> PSCVMDDFRDPQRWKECAKQGKMPCYFDLIEENVYLTERAKNKSHRDIKRMQCECTPLSKDERAQGEIACGEDCLNRLLMIECS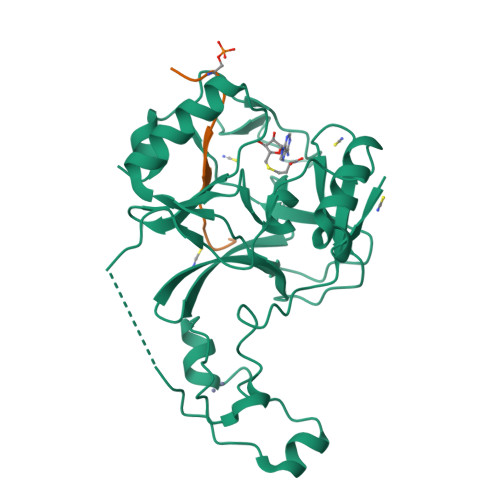SRCPNGDYCSNRRFQRKQHADVEVILTEKKGWGLRAAKDLPSNTFVLEYCGEVLDHKEFKARVKEYARNKNIHYYFMALKNDEIIDATQKGNCSRFMNHSCEPNCETQKWTVNGQLRVGFFTTKLVPSGSELTFDYQFQRYGKEAQKCFCGSANCRGYLGGENRVSIRAAGGK;> APSTGGVMKPHRYR> GAGSMKSSTSKEKVCGENSRHIFNMILNSQRPQFDIKDIGMFHLIDEIERLRKLWKDSEESKKRLNADMREAE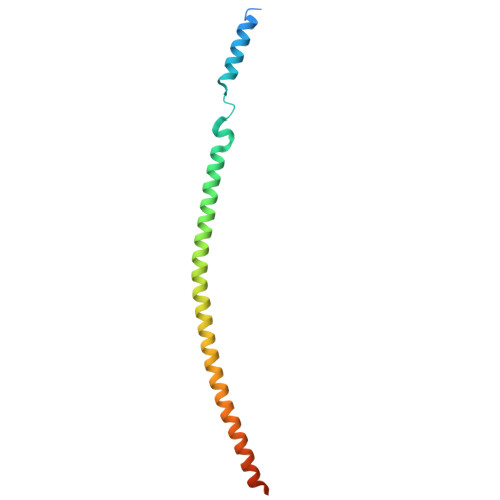EALAKARKKLAMFDIDVKDTQKHLRALMEENKALKLDLNVYETREKQLKDA N-[(3S)-3-methyl-1,1-dioxo-1lambda~6~-thiolan-3-yl]cyclopropanecarboxamide 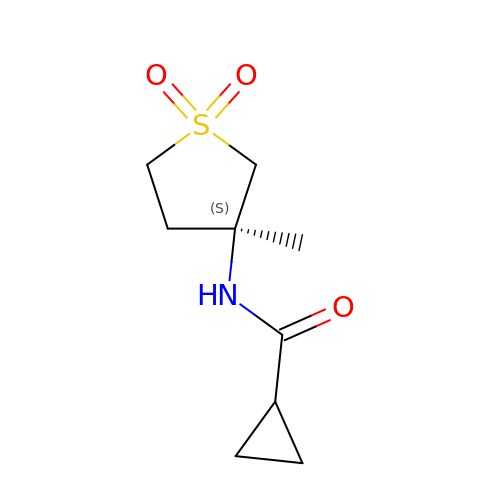| C9 H15 N O3 S | LMUYJJAKMZKBHS-VIFPVBQESA-N>HLVQFNGMIRCTIPGSIPWWDYSDYGCYCGSGGSGTPVDELDRCCQVHDNCYTQAQQLTECSPYSKRYSYDCSEGTLTCKADNDECAAFVC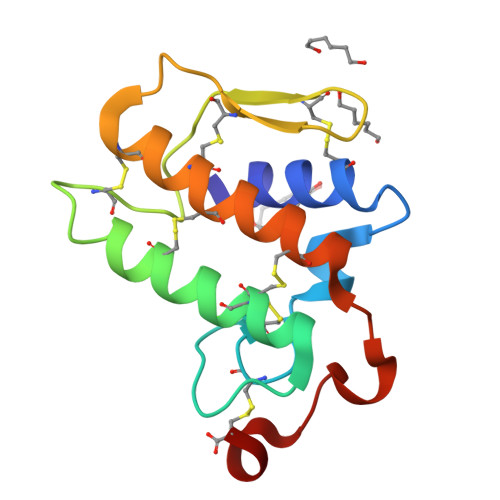DCDRVAAICFAGAPYNKENINIDTTTRC[6x]>MNIIGFSKALFSTWIYYSPERILFDAGEGVSTTLGSKVYAFKYVFLTHGHVDHIAGLWGVVNIRNNGMGDREKPLDVFYPEGNRAVEEYTEFIKRANPDLRFSFNVHPLKEGERVFLRNAGGFKRYVQPFRTKHVSSEVSFGYHIFEVRRKLKKEFQGLDSKEISRLV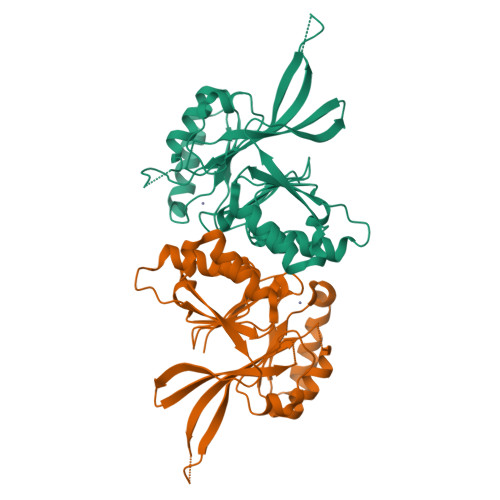KEKGRDFVTEEYHKKVLTISGDSLALDPEEIRGTELLIHECTFLDARDRRYKNHAAIDEVMESVKAAGVKKVILYHISTRYIRQLKSVIKKYREEMPDVEILYMDPRKVFEM[2x]PqsE has two biochemical activities, a protein–protein interaction with RhlR, which increases RhlR transcriptional activity at target promoters, and an esterase activity. Curiously, RhlR function additionally depends on the metallo-β-hydrolase enzyme PqsE, encoded as the final gene in the pqsABCDE biosynthetic operon. With respect to RhlR, PqsE is required to form a protein–protein interaction that enhances the affinity of RhlR for target promoters. The effects of the PqsE E182W and PqsE NI substitutions on pyocyanin production are not through impairment of PqsE catalytic function, as the catalytically inactive variant, PqsE(D73A), remains fully capable of interacting with RhlR and driving pyocyanin production. These results indicate that PqsE has two independent functions, catalysis and interaction with RhlR, and it is interaction with RhlR, not catalysis, that is required for virulence. Moreover, the RhlR–PqsE interaction is essential for P. aeruginosa virulence phenotypes, and therefore, of interest as a focus for antibiotic development.

However, if the morpholine ring is removed and either a phenyl (BB583) or tert-butyl (BB584) group is installed, a modest increase in binding affinity is achieved (EC50 = 71 and 34 nM, respectively). Within that context, BB584 displayed the tightest binding to PqsE and provides a starting scaffold for the design of new derivatives. We determined the crystal structure of BB584 bound to PqsE, which showed a similar orientation in the active site and similar ligand–protein interactions to those observed in the crystal structures of PqsE with BB391 and BB393 bound in the active site. Specifically, the nitrogen on the indazole ring of BB584 bonds with the Fe2 atom, displacing a water molecule that normally resides at this position. Two additional hydrogen bonds exist between BB584 and PqsE sidechains: the BB584 amide oxygen with the hydroxyl group of the S285 sidechain, and the BB584 urea oxygen with the backbone amide N–H of residue Y72. As predicted, the tert-butyl group tucks into the hydrophobic groove that sits between the α-helix consisting of PqsE residues S104-L116 and the backbone of the conserved 69HXHXDH74 motif. Analogous to the structures of BB391 and BB393 bound to PqsE, no significant conformational changes in the protein were induced by binding of BB584 (rmsd of 0.24 Å for 293 Cα atoms), possibly explaining why none of the three compounds disrupt the PqsE–RhlR interaction. In the case of the BB584 ligand, an atomic model of the ligand was fit to the difference electron density observed in the active site of PqsE and refined with partial occupancy (0.93). Thus, it is not surprising that the compounds do not affect the PqsE–RhlR interaction. The crystal structure of the PqsE-BB584 complex solved here provides needed information for launching the structure-guided design of the next generation of molecules targeting the PqsE active site.

> GSHMLRLSAPGQLDDDLCLLGDVQVPVFLLRLGEASWALVEGGISRDAELVWADLCRWVADPSQVHYWLITHKHYDHCGLLPYLCPRLPNVQVLASERTCQAWKSESAVRVVERLNRQLLRAEQRLPEACAWDALPVRAVADGEWLELGPRHRLQVIEAHGHSDDHVVFYDVRRRRLFCGDALGEFDEAEGVWRPLVFDDMEAYLESLERLQRLPTLLQLIPGHGGLLRGRLAADGAESAYTECLRLCRRLLWRQSMGESLDELSEELHRAWGGQSVDFLPGELHLGSMRRMLEILSRQALPLD>SNAESKIKDCPWYDRGFCKHGPLCRHRHTRRVICVNYLVGFCPEGPSCKFMHPRFELPMGTTEQ[4x];>SNAGSINGVPLLEVDLDSFEDKPWRKPGADLSDYFNYGFNEDTWKAYCEKQKRIRMGLEVIPVTSTTNK[8x]

In mammals, the cleavage and polyadenylation specificity factor (CPSF) constitutes the core of the 3′ end processing machinery onto which the remaining factors, including cleavage stimulation factor (CstF) and poly(A) polymerase (PAP), assemble. These interactions are mediated by Fip1, a CPSF subunit characterized by high degree of intrinsic disorder. Here, we report two crystal structures revealing the interactions of human Fip1 (hFip1) with CPSF30 and CstF77. Taken together, these results provide a structural basis for the multivalent scaffolding and regulatory functions of hFip1 in 3′ end processing.

To gain insights into the CPSF30–hFip1 interaction, we determined a crystal structure of a CPSF30 fragment spanning ZF4 and ZF5 domains (CPSF30ZF4–ZF5, residues 118–178) in complex with hFip1CD (residues 138–180 of hFip1 isoform 4) at a resolution of 2.2 Å. The structure reveals that hFip1CD binds CPSF30 in a 2:1 stoichiometry, with one hFip1CD molecule (hFip1CDa) binding predominantly to ZF4 and the other (hFip1CDb) to ZF5. While the overall conformation of the hFip1–CPSF30 complex is highly similar to that of a recent crystal structure of human hFip1–CPSF30, with a root-mean-square deviation of 0.82 Å over the whole complex, in this study, 21 additional residues of hFip1 could be resolved in hFip1CDb due to extended crystallization construct boundaries, with 16 additional residues at the N-terminus (residues 130–145, isoform 4) and 5 additional residues at the C-terminus (residues 177–181, isoform 4). The hFip1CDa–CPSF30 interaction surface (803 Å2) is almost twice as large as the hFip1CDb–CPSF30 interface (478 Å2) because hFip1CDa binds at the ZF4–ZF5 junction and has additional contacts with ZF5. hFip1CDa and hFip1CDb also contact each other directly (215 Å2). ZF4 interaction with hFip1CDa is mediated by a hydrophobic interface centered on Lys127CPSF30 and Phe131CPSF30 and supported by additional salt-bridge contact involving Arg144CPSF30 and Asn159hFip1. In turn, the interaction of ZF5 with hFip1CDb is mainly mediated by Tyr151CPSF30 and Phe155CPSF30 and supported by a salt-bridge contact between Arg168CPSF30 and Asp159hFip1. Interactions with both ZF4 and ZF5 are mediated by a hydrophobic patch in hFip1CD comprising the aromatic side chains of Trp150hFip1, Phe161hFip1, and Trp170hFip1. Moreover, superpositions with CPSF30 ZF2 and ZF3 domains reveal that the interaction surfaces on ZF4 and ZF5 are located on the opposite side of the ZF fold relative to the PAS RNA-binding surfaces of ZF2 and ZF3. We subsequently performed size-exclusion chromatography coupled to multiangle static light scattering (SEC-MALS) to analyze the stoichiometry of hFip1CD–CPSF30ZF4–ZF5 complexes. hFip1CD and wild-type CPSF30ZF4–ZF5 formed a 2:1 complex. In contrast, CPSF30ZF4–ZF5 proteins containing Y127ECPSF30 or F155ECPSF30 mutations formed a 1:1 complex with hFip1CD, while simultaneous mutation of both residues resulted in complete loss of binding.>MHHHHHHENLYFQGAGAGAGAGAMATARELHDVIVETRYGAVRGRSDGTVCVWKGVPFARPPVGPLRFRPPEPPEPWSGVRDATRFGPASVQPEDRLISNLTGGATLPQDEDCLYLNIWSPSPDGRRPVMVWIHGGAYLTGAGSIPWYDGTALAREGDVVVVTLNYRLGALGFLYLEDAFGPEFTGSGNLGILDQIAALRWVRENIAAFGGDPDRVTIFGEAAGAGSVGVLLAAPAARGLFHRAILQSGSGALGVRTAASAARVAARVLQHAGVEPGDREALRSL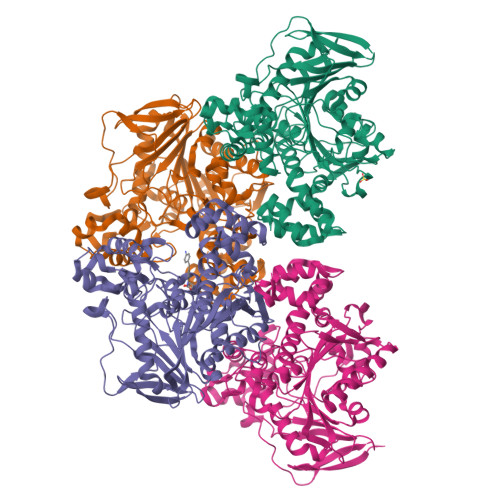PARAWANAVAALGPGLPLGPVVDGTVLPEHPMAALARGAARDVAVLVGVNKDEYNLFALQDPAWLGDDEAALRQRVEAVVGPAAGRLIEFYRSRGEGSLGRRLLPLMSYAVFVRGMLATADAQARVGAPVWAYRFDFETPVLGGVLGACHALEIPFVFNTLDRAGADRFTGTAPERYAVAQAMHRAWIAFAREGNPQHDGLPEWPRYDLEERAVMVFAVEPRVERDPWRAEREVWAAAGVGA[4x]> MKDYDELLKYYELHETIGTGGFAKVKLACHILTGEMVAIRIMDKNTLGSDLPRIKTEIEALKNLRHQHICQLYHVLETANKIFMVLEYCPGGELFDYIISQDRLSEEETRVVFRQIVSAVAYVHSQGYAHRDLKPENLLFDEYHKLKLIAFGLCAKPKGNKDYHLQTCCGSLAYAAPELIQGKSYLGSEADVWSMGILLYVLMCGFLPFDDDNVMALYKKIMRGKYDVPKWLSPSSILLLQQMLQVDPKKRISMKNLLNHPWIMQDYNYPVEWQSKNPFIHLDDDCVTELSVHHRNNRQTMEDLISLWQYDHLTATYLLLLAKKARGKPVRLRLSSFSCGLEHHHHHH

Maternal embryonic leucine zipper kinase (MELK), which is also known as murine protein serine/threonine kinase 38 (MPK38) and pEg3 kinase, is a member of the AMP-activated protein kinase (AMPK)-related kinase family. MELK is a cell cycle-dependent protein kinase that is involved in the regulation of various biological processes, including cell proliferation, spliceosome assembly, hematopoiesis, stem cell self-renewal and apoptosis. [1], [3], [4], [7], [19] and comprises an N-terminal Ser/Thr kinase domain and an adjacent ubiquitin-associated (UBA) domain. However, MELK is unique among these AMPK-related kinases in that it is not activated by LKB1 but undergoes autophosphorylation at the key Thr (Thr167 in human MELK) and additional Ser/Thr residues in the kinase, UBA and TP-rich domains.

All of these kinase-dead mutants were subjected to crystallization trials, and fortunately, the K40R/D150A double mutant yielded crystals with one molecule per asymmetric unit. The structure was determined by molecular replacement and refined to 2.75 Å resolution. This human MELK KD-UBA structure contains residues 2–335, which fold into a kinase domain followed by a noncanonical UBA domain. Notably, the UBA domain of MELK (MELK-UBA) binds to the back of the kinase domain on the opposite face of the catalytic cleft, which is similar to that observed in MARKs but distinct from that in AMPK. Binding of the UBA domain to the kinase domain of MELK results in a buried surface area of more than 1600 Å2, which is significantly larger than that in MARK2 (approximately 1200 Å2). Notably, although the activation segment between and including the DFG and APE motifs is disordered in most inactive kinase structures, this segment (residues 150–178) in our unphosphorylated MELK structure is traceable. The activation segments in the inactive MARK structures are folded into the catalytic cleft between the N- and C-lobes, which hinder the binding of an ATP molecule; in contrast, the activation segment in our unphosphorylated MELK KD-UBA protrudes from the cleft, which allows ATP⋅Mg2+ to bind, and the ordered Gly-rich loop might stabilize the bound ATP. In the structure of the CagA-bound MARK2, the active conformation was induced by the presence of the CagA peptide, which mimics the binding of a typical substrate to the P+1 loop in the kinase domain; however, the P+1 loop in our MELK KD-UBA structure distinctly protrudes, which would obstruct substrate binding. In our MELK structure, three residues of the R-spine in MELK are in perfect configuration as observed in the active MARK2-CagA structure; however, Phe151 adopts a distinct conformation due to the mutation of the preceding Asp150 to Ala. One disulfide bond is intramolecular and formed between Cys154 and Cys168, and the other is intermolecular and formed between two Cys169 residues from symmetry-related molecules.Here, we explore the precise structural inhibitory mechanism of actinonin, which is a slow, tight-binding inhibitor of peptide deformylase (PDF), a metal cation-dependent enzyme. PDF is the first enzyme in the N-terminal methionine excision pathway, an essential and ubiquitous process that contributes to the diversity of N-terminal amino acids. The function of the active-site metal is to activate the reactive water molecule involved in peptide hydrolysis. Actinonin is a natural product with antibiotic activity that inhibits PDF by mimicking the structure of its natural substrates (nascent peptide chains starting with Fo-Met-Aaa, where Fo is a formyl group and Aaa is any amino acid) in their transition state.

The enzyme was observed in two states, a novel open apo-form and a closed, induced, actinonin-bound complex. Binding of actinonin resulted in a tightening of the active site through the collective closure of the entire N-terminal portion of the protein (strands β1, β2, and β3; helix α1; and CD-loop, see Movies S1 and S2, Figure 1C, and Figure S1). The amplitude of the structural change was maximal for Pro60, the Cα of which was shifted 4 Å upon actinonin binding. This collective movement involved the formation of a “super β-sheet” as the result of the large rearrangement of β-strands 4 and 5 relative to the rest of the structure in which actinonin forms an additional strand bridging the two β-sheets (β1 andβ2) on either side of the active site. Hydrogen bonding was also conserved, especially the bond between the backbone nitrogen of Ile42 (corresponding to Ile44 in EcPDF) and the alkyl carbonyl chain of actinonin, which potently contributes to the formation of the super β-sheet (see also below). Between the open and closed states, the side chains of Ile42, Phe58, and Ile130 underwent significant structural changes, corresponding to a hydophobic pocket rearrangement, with Ile42 being the most affected. The closure is very unlikely to result from crystal packing constraints, as soaking the apo-AtPDF crystals in a solution containing actinonin induced the structural transition from the open to the closed state within the crystals without cracking them or altering their diffracting power. The C state is ultimately locked by the super-β-sheet hydrogen bonds extending across the ligand, including those involving Ile42.

>MEIVEYPDPILRAKNKRIDIFDENLKNLVDAMFDVMYKTDGIGLSAPQVGLNVQLMVFNPAGEPGEGKEIVLVNPKIKKYSDKLVPFDEGCLSFPGIYAEVVRPQSVKIDARDITGERFSISLSRLPARIFQHEYDHLEGVLFFDRMTDQVLDSIREELEALEKKYEEKTGLPSPERVEARQKRKAGVGFGKR[2x]> MDAHIANETKQQMTRFAPALVHVIVPDPLLARAGVDPLAPFAAHAQTRYHGSGVCEPWVSVFAGHVQTGAVESVLTLPPLQRPRGPGGLFVSLPLALGAHFDGFTTAALRVGARELVFTYDELLPARTRYNVDGERLERLCRQFANYARARRVAPAVAAAGGHIDALLPPAAATIDGEAQLTRGGFDDPAAPHARDADREILSLVRRAAELVAARHPVRSHVASGLMQGALARRGGGGDGAGALEAAATVPAPAAREDANGGGAAWRDELLLTPQDPRPLTALDWLDAGYAALAGGDAPAHVWRRRPVSLVARRHYQTGETFVVVAYEHSTAWGGRRGPRGEPLARVLAEECERHGVEHPRALPAEARRELVRRHAELAVPLGDEEPPLPVFDATAELVLLERFRNACVRALLAGVRE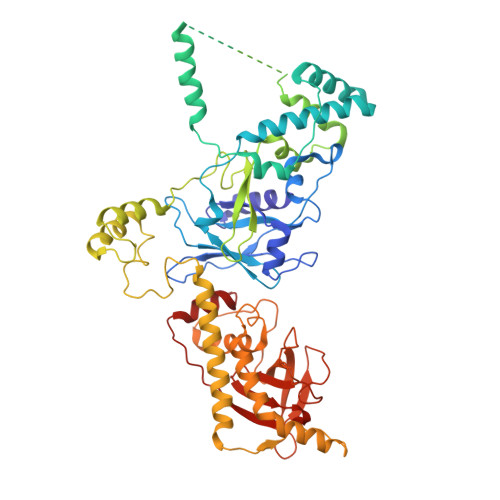SVRREPRMRQIIEFAIRPRDREAVLDVAGRAPALLDAFARRLEHTPAREMVDSGLMTAAAAHLAARATAGYVTFESGPLLGGVFLFDYYSAGGEVIRVTRAPLAVAVEPATRGQFACRFRGASHRCLPGESYAYLCVGVSRDLRALVVLPGGFGFFATLRLEWPAALVDPVLERLCRRV> HHHHHHRQYNLVTRESLPQALRRIEEAKRIALDTETTGLQIYLPGFELVGLAVAVSPEEAYYFPYAHRDFAGLRYQPENLSREDLLRVLELAFQRSVVYHNAAYDRQVLYRTLGIPFERS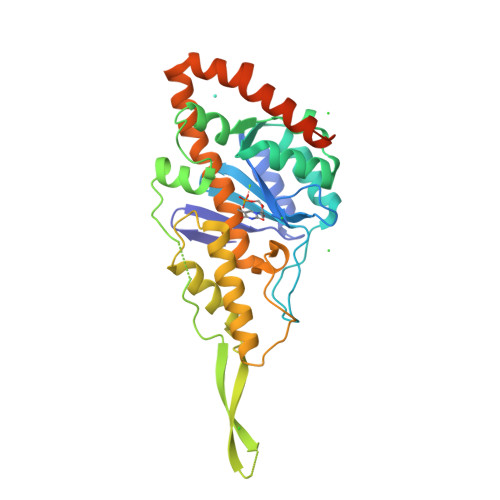YGNDTMIALHLMDENHSNSLKEWSKTLLGLEESMAVPELPSLTDVELVDTVNKSGRKYKKKVHKLAPDWLDRLKTAFLSVHNGGVSFAALHKLVAQAFNTLKARGILYYPGSFPVDFRYFHVHLAHIYALDDAMNTLALWEHVEIFLQLHPQLERLYLDIELPVNDIMTRASARGVLVDRSVIERIEADLQAKLEERE>[2x]MNYSIRLFKIMGIPIELHITFILFLVVIIGLSIMNN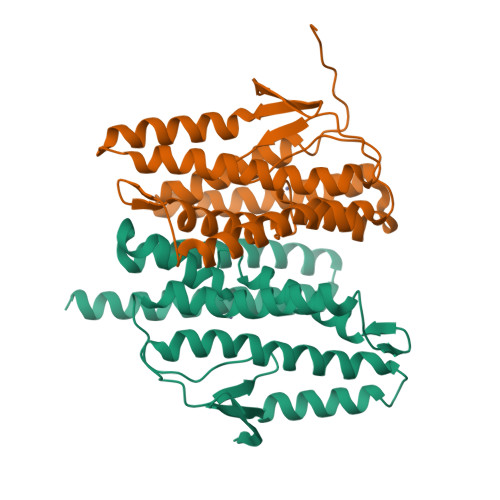SIFWAVLFILLFVSVVLHELGHSYVAKKYGVKIEKILLLPIGGVAMMDKIPKEGELRIGIAGPLVSFIIGIVLLIVSQFFDININGYPLLYTLSLLNLMLGGFNLIPAFPMDGGRILRAILSKKYGYLKSTKIAANIGKSLALIMLLFGLLSMNIILILVSLFVYFGAEQESRVVEVETIFKNIKAKD> MLPRETDEEPEEPGRRGSFVEMVDNLRGKSGQGYYVEMTVGSPPQTLNILVDTGSSN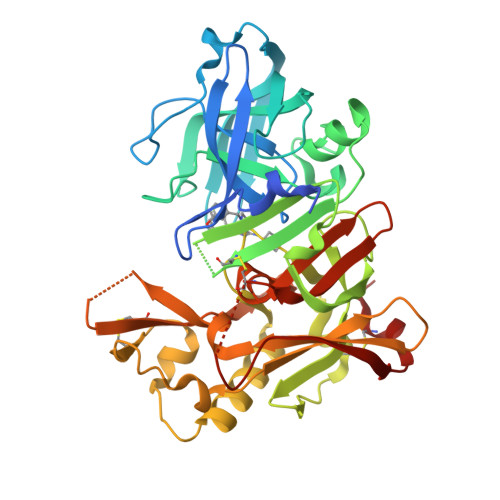FAVGAAPHPFLHRYYQRQLSSTYRDLRKGVYVPYTQGAWAGELGTDLVSIPHGPNVTVRANIAAITESDKFFINGSNWEGILGLAYAEIARPDDSLEPFFDSLVKQTHVPNLFSLQLCGAGFPLNQSEVLASVGGSMIIGGIDHSLYTGSLWYTPIRREWYYEVIIVRVEINGQDLKMDCKEYNYDKSIVDSGTTNLRLPKKVFEAAVKSIKAASSTEKFPDGFWLGEQLVCWQAGTTPWNIFPVISLYLMGEVTNQSFRITILPQQYLRPVEDVATSQDDCYKFAISQSSTGTVMGAVIMEGFYVVFDRARKRIGFAVSACHVHDEFRTAAVEGPFVTLDMEDCGYN>[2x]MIGVLLMKSRANEEYGLRLGSQIFVKEMTRTGLATKD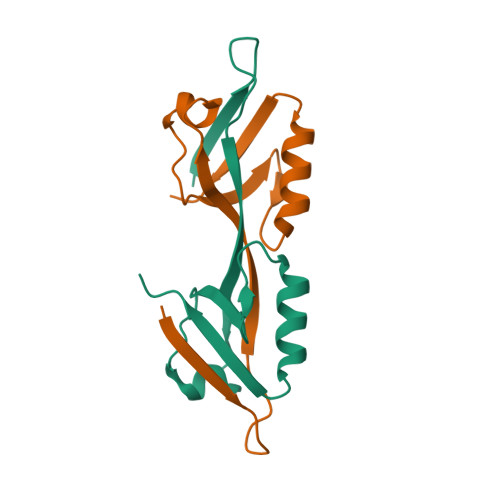GNLHEGDIILKINGTVTENMSLTDARKLIEKSRGKLQLVVLRDLEHHHHHH>MAQVINTNSLSLLTQNNLNKSQSALGTAIERLSSGLRINSAKDDAAGQAIANRFTANIKGLTQASRNANDGISIAQTTEGALNEINNNLQRVRELAVQSANSTNSQSDLDSIQAEITQRLNEIDRVSGQTQFNGVKVLAQDNTLTIQVGANDGETIDIDLKQINSQTLGLDTLNVQQKYKVSDTAATVTGYADTTIALDNSTFKASATGLGGTDQKIDGDLKFDDTTGKYYAKVTVTGGTGKDGYYEVSVDKTNGEVTLAGGATSPLTGGLPATATEDVKNVQVANADLTEAKAALTAAGVTGTASVVKMSYTDNNGKTIDGGLAVKVGDDYYSATQNKDGSISINTTKYTADDGTSKTALNKLGGADGKTEVVSIGGKTYAASKAEGHNFKAQPDLAEAAATTTENPLQKIDAALAQVDTLRSDLGAVQNRFNSAITNLGNTVNNLTSARSRIEDSDYATEVSNMSRAQILQQAGTSVLAQANQVPQNVLSLLR[17x];>MASISSLGVGSNLPLDQLLTDLTKNEKGRLTPITKQQSANSAKLTAYGTLKSALEKFQTANTALNKADLFKSTVASSTTEDLKVSTTAGAAAGTYKINVT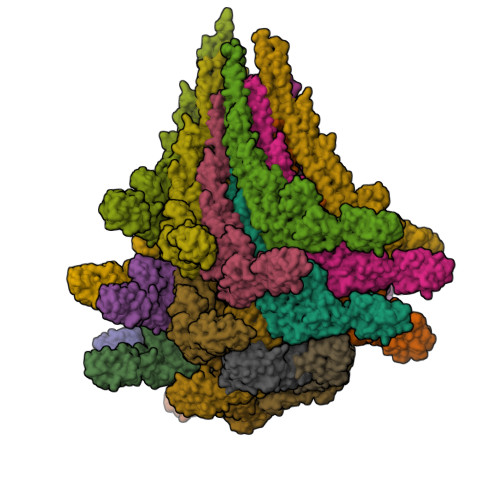QLAAAQSLATKTTFATTKEQLGDTSVTSRTIKIEQPGRKEPLEIKLDKGDTSMEAIRDAINDADSGIAASIVKVKENEFQLVLTANSGTDNTMKITVEGDTKLNDLLAYDSTTNTGNMQELVKAENAKLNVNGIDIERQSNTVTDAPQGITLTLTKKVTDATVTVTKDDTKAKEAIKSWVDAYNSLVDTFSSLTKYTAVEPGEEASDKNGALLGDSVVRTIQTGIRAQFANSGSNSAFKTMAEIGITQDGTSGKLKIDDDKLTKVLKDNTAAARELLVGDGKETGITTKIATEVKSYLADDGIIDNAQDNVNATLKSLTKQYLSVSNSIDETVARYKAQFTQLDTMMSKLNNTSSYLTQQFTAMNKS[5x]>MSNMNQTIMDAFHFRHATKQFDPQKKVSKEDFETILESGRLSPSSLGLEPWKFVVIQDQALRDELKAHSWGAAKQLDTASHFVLIFARKNVTSRSPYVQHMLRDIKKYEAQTIPAVEQKFDAFQADFHISDNDQALYDWSSKQTYIA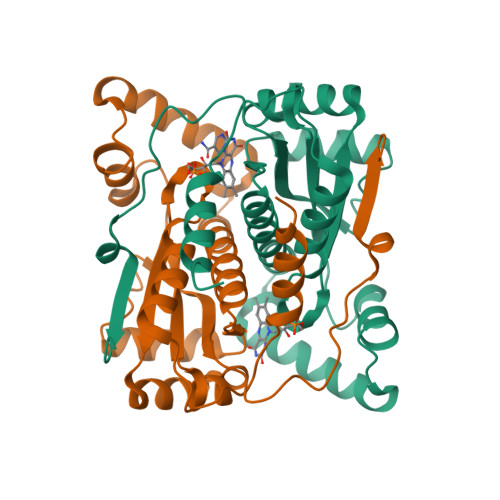LGNMMTTAALLGIDSCPMEGFSLDTVTDILANKGILDTEQFGLSVMVAFGYRQQDPPKNKTRQAYEDVIEWVGPKE[5x]>[2x]GSMSAPDSITVTVADHNGVAVLSIGGEIDLITAAALEEAIGEVVADNPTALVIDLSAVEFLGSVGLKILAATSEKI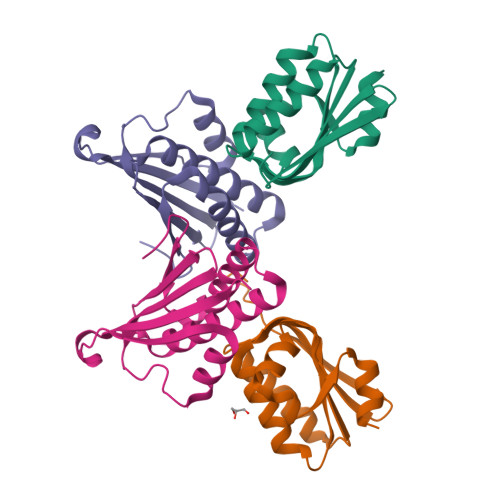GQSVKFGVVARGSVTRRPIHLMGLDKTFRLFSTLHDALTGVRGGRIDR;>[2x]MADSDLPTKGRQRGVRAVELNVAARLENLALLRTLVGAIGTFEDLDFDAVADLRLAVDEVCTRLIRSALPDATLRLVVDPRKDEVVVEASAACDTHDVVAPGSFSWHVLTALADDVQTFHDGRQPDVAGSVFGITLTARRAASSR Interhelical interactions between side chains of residues at the e and g positions as well as the packing of these amino acids against the hydrophobic a and d core residues also contribute significantly to oligomerization-state specificity of coiled coils. This is exemplified by the trimerization motif Arg(g)-h(a)-x-x-h(d)-Glu(e) (denoted R-hxxhE where h(a) = Ile, Leu, Val, Met; h(d) = Leu, Ile, Val; x = any amino acid residue) that specifies a three-stranded, parallel topology of coiled-coil domains. The trimerization driving force of the motif can be explained by optimal side chain–side chain interactions whereby the strictly conserved arginine and glutamate residues form a distinct, bifurcated, interhelical salt-bridge network and participate in the formation of the hydrophobic core by establishing tight packing interactions to the neighbouring residues at the a and d positions through their aliphatic moieties. Because of its substantial size of 18 continuous heptad repeats, we used a combination of trimer-specific determinants to switch the cortexillin-1 coiled coil from a dimer to a trimer. Accordingly, we rationally substituted residues to complement two ideal trimerizer motifs of the type R-IxxIE and introduced one additional hydrophobic core isoleucine residue in the trigger sequence of the cortexillin-1 coiled coil (referred to as Cort-Ir-M1).

Because high-resolution structural information could not be obtained for the full-length Cort-Ir-M1 trimer, the aim of the present study was to perform a detailed structural characterization of two fragments spanning the trigger sequence of the trimeric Cort-Ir-M1 coiled coil using circular dichroism, anatytical ultracentrifugation and x-ray crystallography. As expected, the peptide forms a trimer with characteristics typical of left-handed parallel coiled coils. Accordingly, the conformations of side chains and the position of the water molecule between Arg7 and Glu12, and Arg14 and Glu19 can be superimposed almost perfectly onto the trimerization motifs of the coronin-1 coiled coil, ccβ and GCN4p-M3, demonstrating structural conservation of the motif (not shown). Tight interhelical hydrophobic contacts involve the side chain of Ile8′ at position a′ of the first trimerization motif, which is optimally shielded from solvent exposure by the aliphatic side-chain portion of Arg7. In the structure, the five introduced isoleucine residues can be accommodated in the most preferred rotamer at the hydrophobic core positions. Accordingly, the acute packing geometries of the five isoleucine residues are very similar to those seen in the crystal structure of the trimeric GCN4-pII variant, in which all a and d positions are occupied by isoleucine residues (not shown). Notably, a similar optimal packing of the hydrophobic core and the presence of an extensive network of surface salt bridges are typically observed in thermostable proteins.

>[12x]GSLELIKLRIMEIEARIAKIEKDRAIL>[4x]MNQNLLVTKRDGSTERINLDKIHRVLDWAAEGLHNVSISQVELRSHIQFYDGIKTSDIHETIIKAAADLISRDAPDYQYLAARLAIFHLRKKAYGQFEPPALYDHVVKMVEMGKYDNHLLEDYTEEEFKQMDTFIDHDRDM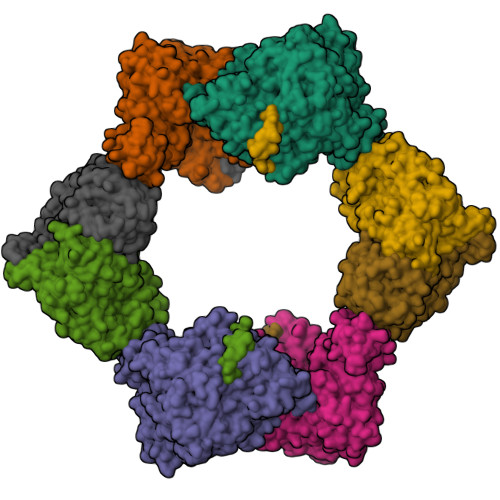TFSYAAVKQLEGKYLVQNRVTGEIYESAQFLYILVAACLFSNYPRETRLQYVKRFYDAVSTFKISLPTPIMSGVRTPTRQFSSCVLIECGDSLDSINATSSAIVKYVSQRAGIGINAGRIRALGSPIRGGEAFHTGCIPFYKHFQTAVKSCSQGGVRGGAATLFYPMWHLEVESLLVLKNNRGVEGNRVRHMDYGVQINKLMYTRLLKGEDITLFSPSDVPGLYDAFFADQEEFERLYTKYEKDDSIRKQRVKAVELFSLMMQERASTGRIYIQNVDHCNTHSPFDPAIAPVRQSNLCLEIALPTKPLNDVNDENGEIALCTLSAFNLGAINNLDELEELAILAVRALDALLDYQDYPIPAAKRGAMGRRTLGIGVINFAYYLAKHGKRYSDGSANNLTHKTFEAIQYYLLKASNELAKEQGACPWFNETTYAKGILPIDTYKKDLDTIANEPLHYDWEALRESIKTHGLRNSTLSALMPSETSSQISNATNGIEPPRGYVSIKASKDGILRQVVPDYEHLHDAYELLWEMPGNDGYLQLVGIMQKFIDQSISANTNYDPSRFPSGKVPMQQLLKDLLTAYKFGVKTLYYQNTRDGAEDAQDDLVPSIQDDGCESGACKI;>AYTTFSQTKNDQLKEPMFFGQPVNVARYDQQKYDIFEKLIEKQLSFFWRPEEVDVSRDRIDYQALPEHEKHIFISNLKYQTLLDSIQGRSPNVALLPLISIPELETWVETWAFSETIHSRSYTHIIRNIVNDPSVVFDDIVTNEQIQKRAEGISSYYDELIEMTSYWHLLGEGTHTVNGKTVTVSLRELKKKLYLCLMSVNALEAIRFYVSFACSFAFAERELMEGNAKIIRLIARDEALHLTGTQHMLNLLRSGADDPEMAEIAEECKQECYDLFVQAAQQEKDWADYLFRDGSMIGLNKDILCQYVEYITNIRMQAVGLDLPFQTRSNPIPWINTWLVSDNVQVAPQEVEVSSYLVGQIDSEVDTDDLSNFQL[4x]> MIAPMEKLVLAGPKGRAKELLQSLQQAGVVHLETLRPEALSAYQLSPEERAELRRWEAVSAGAEHTLSLLGLEAEPARPFPEGLEAAEKALSPIQAHAEGLTRQKQELEEELALAQAYLEPLERLAALAHGLDKSPFLRVIPFLLTEKELPLVEEALRKALEDRYLLAHEAYAGGVAALVVVHRKEVDQAKAALSRAGVAELRLPGALGELPLSEAARRLKERAEAAPRELSEVRQHLAKLARESASTLQSLWTRAQDEVARLKALEELASGRFGFALLGYVPVKAKPKVEEALARHKESVVYAFEPVDEHHEADRIPVVLDNPPWAKPFELLVSFLNTPKYGTFDPTPVVPVFFPFWFGMIVGDIGYALLFYLVGRWLSGYVKRNEPLVIDLFALKLKPQVIGKLVHILNWMVFWTVVWGVIYGEFF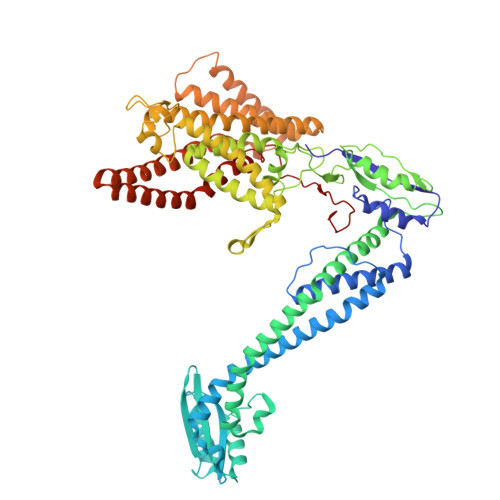GTFLEHLGVFGTPEHPGLIPILIHRIDTAKTANLLILLSVAFGVVLVFFGLALRAYLGLKHRHMAHFWEGVGYLGGLVGVLALAASYLGNLQAGWLQGLMYLGFGVFLLAVLMSRIWLMIPEIFTQAGHILSHIRIYAVGAAGGILAGLLTDVGFALAERLGLLGVLLGLLVAGVLHLLILLLTTLGHMLQPIRLLWVEFFTKFGFYEENGRPYRPFKSVREAQ>[2x]MSTRKAVIGYYFIPTNQINNYTETDTSVVPFPVSNITPAKAKQLTHINFSFLDINSNLECAWDPATNDAKARDVVNRLTALKAHNPSLRIMFSIGGWYY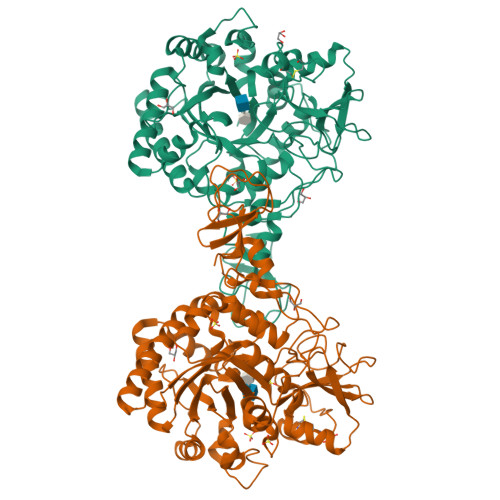SNDLGVSHANYVNAVKTPASRAKFAQSCVRIMKDYGFDGVDIDWEYPQAAEVDGFIAALQEIRTLLNQQTITDGRQALPYQLTIAGAGGAFFLSRYYSKLAQIVAPLDYINLMTYDLAGPWEKVTNHQAALFGDAAGPTFYNALREANLGWSWEELTRAFPSPFSLTVDAAVQQHLMMEGVPSAKIVMGVPFYGRAFKGVSGGNGGQYSSHSTPGEDPYPSTDYWLVGCEECVRDKDPRIASYRQLEQMLQGNYGYQRLWNDKTKTPYLYHAQNGLFVTYDDAESFKYKAKYIKQQQLGGVMFWHLGQDNRNGDLLAALDRYFNAADYDDSQLDMGTGLRYTGVGPGNLPIMTAPAYVPGTTYAQGALVSYQGYVWQTKWGYITSAPGSDSAWLKVGRVA>MSESPLRLDRLRDFVSALGELLDRHPDEESVLREGRSLLGELVRHDDWLPEEFAQPDPERYQQYLLHADSRQRFSVVSFVWGPGQTTPVHDHRVWGLIGMLRGAEDAQSFELGAEGLRPIGDPVRLSPGQVEAVSPRIGDIHRVFNASPDQPSISIHVYGANIGAVRRAVYLPDGSEKPFISGYSNQFLPNIWDQSKESARPVDLVPR[4x]

Thiol dioxygenases are a subset of nonheme iron oxygenases that catalyze the formation of sulfinic acids from sulfhydryl-containing substrates and dioxygen. Av3MDO exhibits the classic thiol dioxygenase cupin fold consisting of three N-terminal alpha-helices followed by a series of 11 β-strands forming the cupin β-barrel structure that houses the enzymatic active site. Like in Pa3MDO and other thiol dioxygenases, the iron center of Av3MDO is coordinated by three His residues (90, 92, and 142) contained within the conserved cupin motifs. The moderately hydrophobic dimer interface buries an average of ∼1260 Å2 (1199–1322 Å2 depending on the specific dimer pair) or ∼13% of the total monomer surface area and is structurally similar to the dimers observed for 3MDOs from other bacteria, all suggesting that it represents a physiologically relevant assembly.

Because intrinsic structural differences between Av3MDO and Pa3MDO are expected to be small owing to their high sequence similarity, we considered the possibility that the observed active site differences could arise from the bound substrate mimetic in Av3MDO. To test this hypothesis, we identified alternative crystallization conditions to allow investigation of the resting-state structure of Av3MDO. Following further sparse matrix screening, we identified a crystallization condition containing a nonpolyacrylate precipitant (pentaerythritol propoxylate) as well as sodium thiocyanate that produced yellowish, rod-shaped crystals. The crystals diffracted X-rays to ∼3 Å resolution and belonged to space group P6122 with a pair of dimers (same conserved interface described above) in the asymmetric unit. Strong difference density in the equatorial positions of the iron center was adequately explained by two water molecules while the axial position contained an elongated difference peak that was too strong to represent only water or chloride. Placement of thiocyanate, a well-known Fe(III)-binding ligand present at > 0.3 M concentration in the crystal mother liquor, at this position adequately accounted for the density with reasonable refined B-factors. Analysis of difference maps and refined B-factors provided strong evidence that coordination is through the nitrogen atom, which is consistent with the coordination preferences of Fe(III), a hard Lewis acid, and small-molecule crystallography results for high-spin, nonheme iron model compounds. Contrary to our hypothesis, we observed that the active site has maintained its closed state in this new crystal form. By contrast, the conformation of Trp81 is identical in every copy within the asymmetric units of the two Av3MDO structures, suggesting it represents an intrinsic structural difference as compared with Pa3MDO. A notable finding from our structural analysis of Av3MDO was its lack of a patent tunnel for substrate diffusion to the active site. This observation was consist across all crystallographically independent protomers of both Av3MDO crystal forms.> STPAITLENPDIKYPLRLIDKEVVNHDTRRFRFALPSPEHILGLPVGQHIYLSARIDGNLVIRPYTPVSSDDDKGFVDLVIKVYFKDTHPKFPAGGKMSQYLESMKIGDTIEFRGPNGLLVYQGKGKFAIRPDKKSSPVIKTVKSVGMIAGGTGITPMLQVIRAIMKDPDDHTVCHLLFANQTEKDILLRPELEELRNEHSARFKLWYTVDRAPEAWDYSQGFVNEEMIRDHLPPPEEEPLVLMCGPPPMIQYACLPNLERVGHP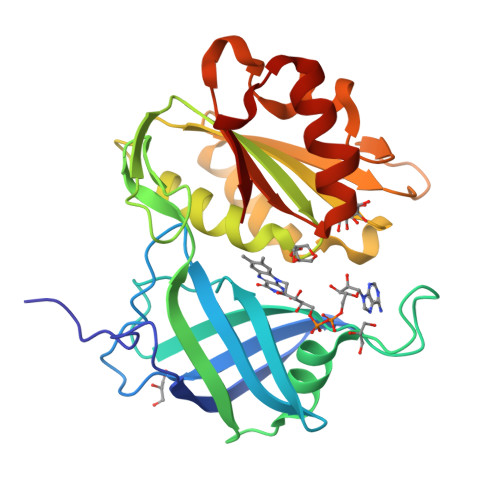KERCFAF>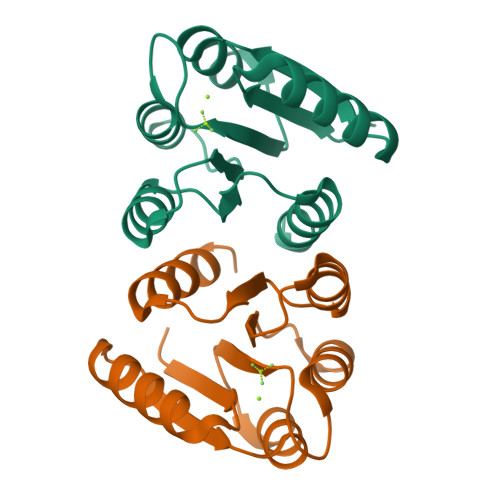[8x]MGHHHHHHTQILIVEDEQNLARFLELELTHENYNVDTEYDGQDGLDKALSHYYDLIILDLMLPSINGLEICRKIRQQQSTPIIIITAKSDTYDKVAGLDYGADDYIVKPFDIEELLARIRAILRRQPQ4-OXORETINOL | C20 H28 O2 | 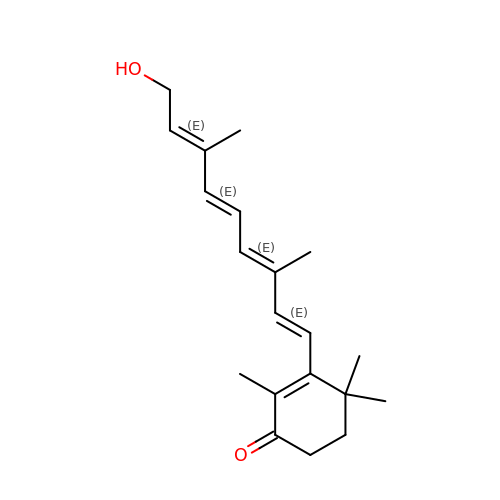PLIUCYCUYQIBDZ-RMWYGNQTSA-N> KWTPPRSPFNLVQETLFHDPWKLLIATIFLNRTSGKMAIPVLWKFLEKYPSAEVARTADWRDVSELLKPLGLYDLRAKTIVKFSDEYLTKQWKYPIELHGIGKYGNDSYRIFCVNEWKQV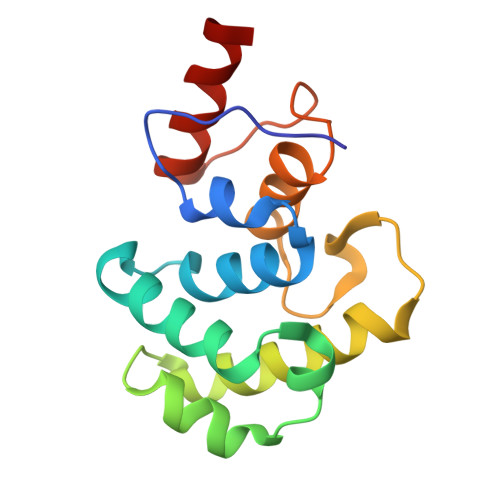HPEDHKLNKYHDWLWENH>MANKPTQPLFPLGLETSESSNIKGFNNSGTIEHSPGAVMTFPEDTEVTGLPSSVRYNPDSDEFEGYYENGGWLSLGGGGIRWETLPHAPSSNLLEGRGYLINNTTGTSTVVLPSPTRIGDSVTICDAYGKFATYPLTVSPSGNNLYGSTEDMAITTDNVSATFTWSGPEQGWVITSGVGLGQGRVYSREIFTQILASETSAVTLNTPPTIVDVYADGKRLAESKYSLDGNVITFSPSLPASTELQVIEYTPIQLGNGGGSGSSTITWVYNGGSAI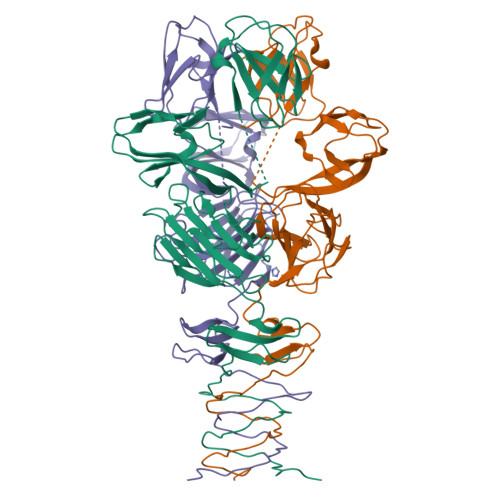GGETEITLDIVVDDVPAIDINGSRQYKNLGFTFDPLTSKITLAQELDAEDEVVVIINGTPHHHHHH[2x]>CSRLVTETQYGTMLMRTADWVSTAPFDGHMSVFPVGTERTMRGQVAEYQQAMTKWQTKYHTLSIEEHGAFGGLSGQTSNEKGLSVMALSQHDSEPYLSQHKDNGAPAVNTADVVSFITERYATTAEVKAALDNGEFQIAWASAPNGMEHAAPLHYSVVDADGNIMLIQLVKGGEQKIYLGDAESDLRVKTNDPLQEKHREYMQQFDLKDPSVATKMPWSIGGLERNSRLLAMSTHMDLEGLSYTETVARQKGTFDAAALVPFGVQDPKTGEDYPSFFSMQYNLDNGDIWFRSLMSGKEIKFNLEDTKQFKTPMHADIMAQVDKGAQTITWSKMHHHHH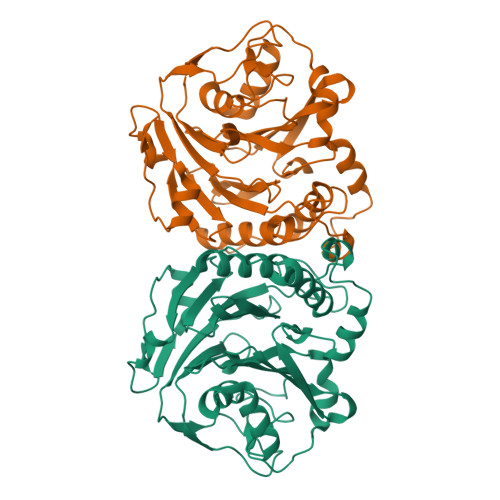H[2x]> MMIVIMDNGGQYVHRIWRTLRYLGVETKIIPNTTPLEEIKAMNPKGIIFSGGPSLENTGNC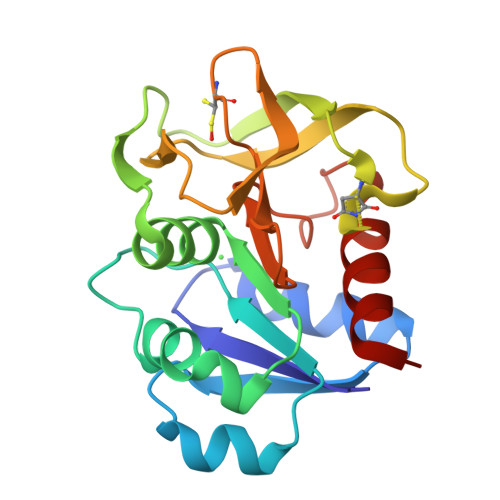EKVLEHYDEFNVPILGICLGHQLIAKFFGGKVGRGEKAEYSLVEIEIIDENEIFKGLPKRLKVWESHMDEVKELPPKFKILARSETCPIEAMKHEELPIYGVQFHPEVAHTEKGEEILRNFAKLCGEL> DGKIDLETPDSILASTNLRALLNKQTFSLLPPLYQYNLIQLLPSVDREASELEQPSSSASGGSPSEAIRLSASCLNNEFFARACLEWRERLSEGE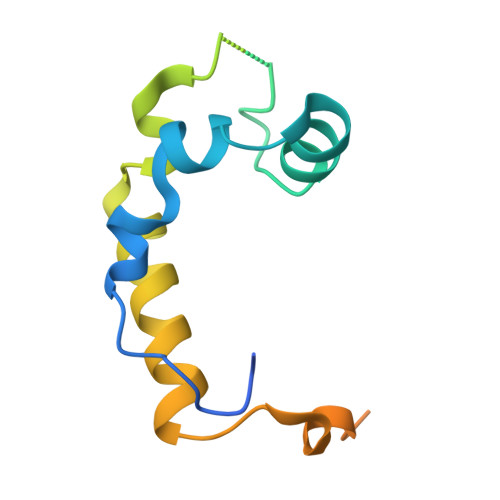FTPENQLKLKTEAEREKNKLDPWKLKHFEPFWGEKNSRG> MIEDEMSREQIIKDGGNILVTAGAGSGKTTILVSKIEADLKENKTHYSIAAVTFTNKAAKEIEGRLGYSSRGNFIGTNDGFVESEIIRPFIKDAFGNDYPDNFTAEYFDNQFASYDKGLQVLK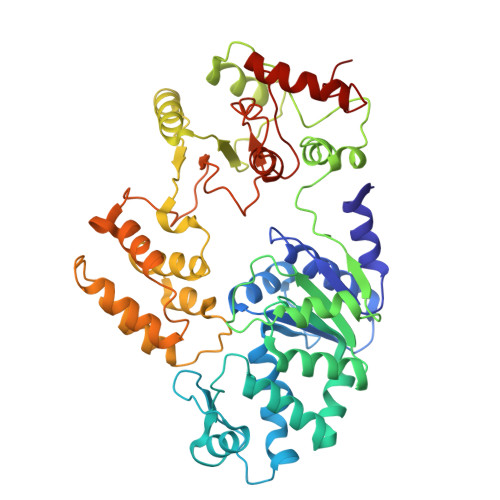YQNILGTYSNPKKNFKFQLALDILKKSLVARQYIFSKYFKIFIDEYQDSDKDMHNLFMYLKDQLKIKLFIVGDPKQSIYIWRGAEPENFNGLIENSTDFNKYHLTSNFRCCQDIQNYSNLFNEETRSLIKEKNEVQNVISIADDMPISDILLKLTEEKQVLNIEAELVILVRRRNQAIEIMKELNEEGFNFIFIPQTPLDRATPNATLLKEVIKYVKNDRYSIYDLAAEIVGNLSSREIKEIQKIINELLVPNINQVLINQVLINLFAKLEITLDTREITAFTEVMMTNEFDIAFDTNEYLHKIFTVHSAKGLEFNQVIITASDYNVHYNRDTNEHYVATTRAKDKLIVIMDNKKYSDYIETLMKELKIKNIIKSI N,N-dimethylmorpholine-4-sulfonamide | 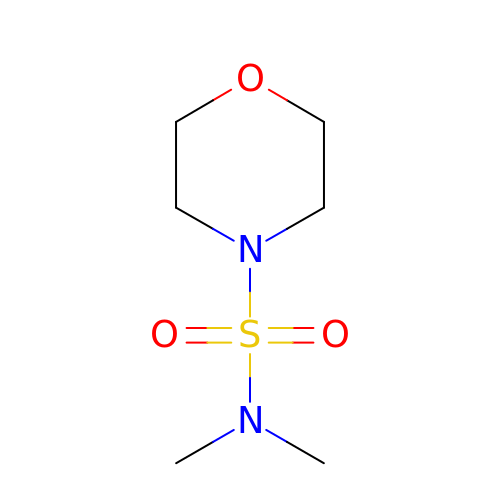C6 H14 N2 O3 S | OPFOHHASSCNHHQ-UHFFFAOYSA-N(2R,3E)-2-[(2S,3R,6S)-2,3-bis(4-chlorophenyl)-6-(4-fluorobenzyl)-5-oxomorpholin-4-yl]pent-3-enoic 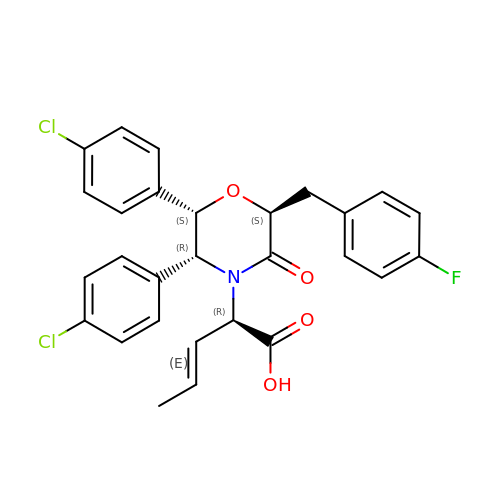acid | C28 H24 Cl2 F N O4 | KFJHASQDDHBQDA-GYEZOCHYSA-N> DLKFKRHKNKHIQGFPTLGERLDNLQDIKKA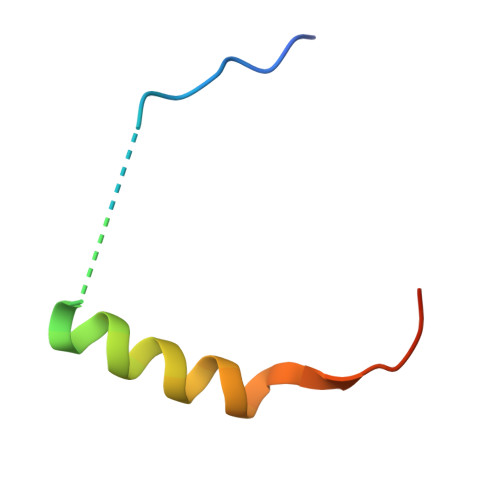KRVENFNSS> MAEHVVYVGNKPVMNYVLATLTQLNEGADEVVIKARGRAISRAVDVAEIVRNRFMPGVKVKEIKIDTEELE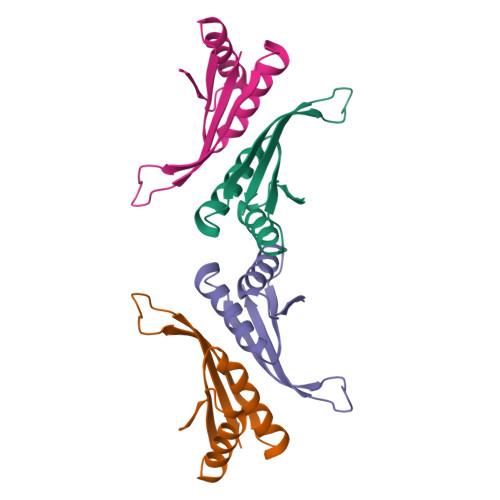SEQGRRSNVSTIEIVLAK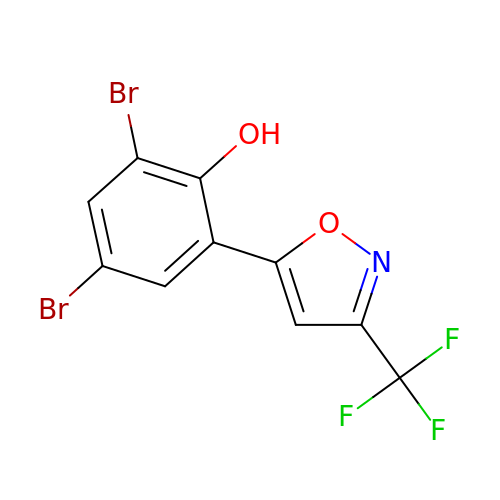2,4-bis(bromanyl)-6-[3-(trifluoromethyl)-1,2-oxazol-5-yl]phenol | C10 H4 Br2 F3 N O2 | UPPPIWMLZRPTQQ-UHFFFAOYSA-N>[2x]DEIDLSALRDPAGIFELVELVGNGTYGQVYKGRHVKTGQLAAIKVMDVTGDEEEEIKQEINMLKKYSHHRNIATYYGAFIKKNPPGMDDQLWLVMEFCGAGSVTDLIKNTKGNTLKEEWIAYICREILRGLSHLHQHKVIHRDIKGQNVLLTENAEVKLVDFGVSAQLDRTVGRRNTFIGTPYWMAPEVIACDENPDATYDFKSDLWSLGITAIEMAEGAPPLCDM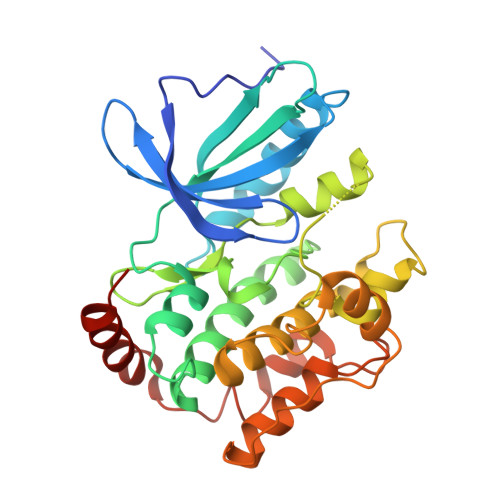HPMRALFLIPRNPAPRLKSKKWSKKFQSFIESCLVKNHSQRPATEQLMKHPFIRDQPNERQVRIQLKDHIDRTKKKRG>[4x]CSSLSIRTTDDKSLFARTMDFTMEPDSKVIIVPRNYGIRLLEKENVVINNSYAFVGMGSTDITSPVLYDGVNEKTYADEPKKGTGLMGAMLYYATFATYADEPKKGTTGINPVYVISQVLGNCVTVDDVIEKLTSYTLLNEANIILGFAPPLHYTFTDASGESIVIEPDKTGITIHRKTIGVMTNSPGYEWHQTNLR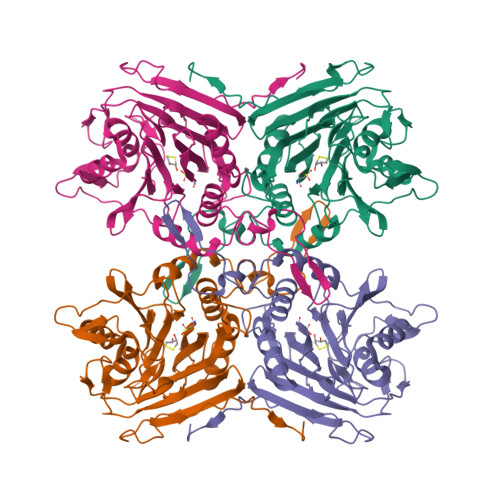AYIGVTPNPPQDIMMGDLDLTPFGQGAGGLGLPGDFTPSARFLRVAYWKKYTEKAKNETEGVTNLFHILSSVNIPKGVVLTNEGKTDYTIYTSAMCAQSKNYYFKLYDNSRISAVSLMAENLNSQDLITFEWDRKQDIKQLNQVNVMS> EKLGDICFSLRYVPTAGKLTVVILEAKNLKKMDVGGLSDPYVKIHLMQNGKRLKKKKTTIKKNTLNPYYNESFSF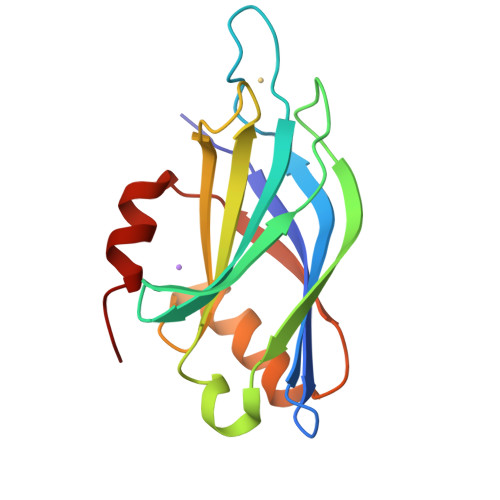EVPFEQIQKVQVVVTVLDYDKIGKNDAIGKVFVGYNSTGAELRHWSDMLANPRRPIAQWHTLQVEEEVDAMLAVKK>[2x]MSSKANHAKTVICGIINVTPDSFSDGGQFFALEQALQQARKLIAEGASMLDIGGESTRPGSSY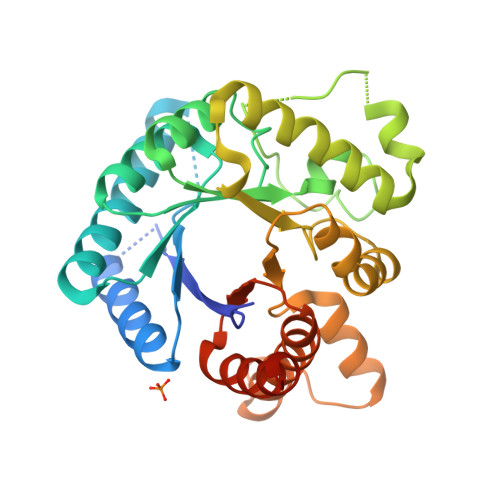VEIEEEIQRVVPVIKAIRKESDVLISIDTWKSQVAEAALAAGADLVNDITGLMGDEKMPHVVAEARAQVVIMFNPVMARPQHPSSLIFPHFGFGQAFTEEELADFETLPIEELMEAFFERALARAAEAGIAPENILLDPGIGFGLTKKENLLLLRDLDKLHQKGYPIFLGVSRKRFVINILEENGFEVNPETELGFRNRDTASAHVTSIAARQGVEVVRVHDVASHRMAVEIASAIRLADEAENLDLKQYK> MAQLKKKLQALKKKNAQLKWKLQALK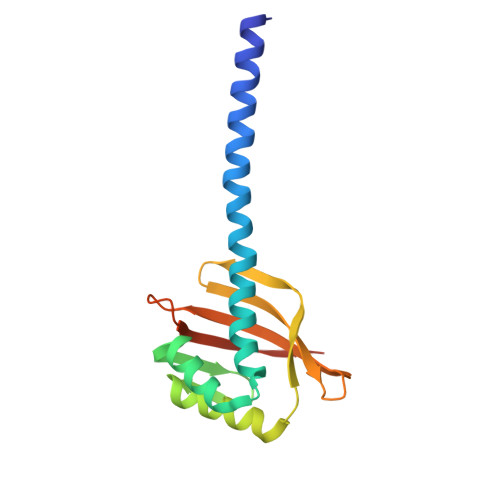KKLAQATQHLTIAQTYLAAWNEEDNERRRHLVGQAWAENTRYVDPLMQGEGQQGIAAMIEAARQKFPGYRFVLAGTPDGHGNFTRFSWRLISPDGDDVAGGTDVVSLNTEGRIDNVVGFLDGAVSHHHHHH> QSACTLQS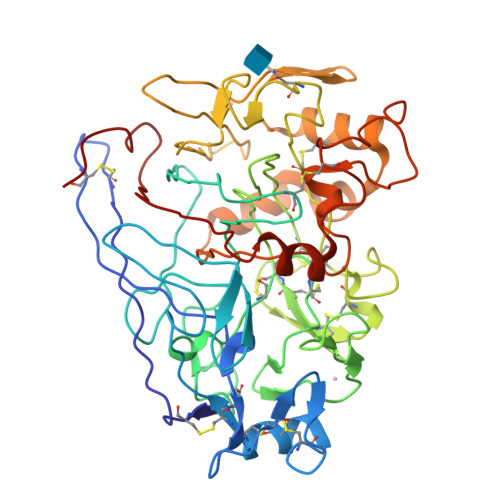ETHPPLTWQKCSSGGTCTQQTGSVVIDANWRWTHATNSSTNCYDGNTWSSTLCPDNETCAKNCCLDGAAYASTYGVTTSGNSLSIDFVTQSAQKNVGARLYLMASDTTYQEFTLLGNEFSFDVDVSQLPCGLNGALYFVSMDADGGVSKYPTNTAGAKYGTGYCDSQCPRDLKFINGQANVEGWEPSSNNANTGIGGHGSCCSEMDIWEANSISSHVAPHPCTTVGQEICEGDGCGGTYSDNRYGGTCDPDGCGWNPYRLGNTSFYGPGSSFTLDTTKKLTVVTQFETSGAINRYYVQNGVTFQQPNAELGSYSGNELNDDYCTAEEAEFGGSSFSDKGGLTQFKKATSGGMVLVMSLWDDYYANMLWLDSTYPTNETSSTPGAVRGSCSTSSGVPAQVESQSPNAKVTFSNIKFGPIGSTGNPSG PRPP is formed from ATP and D-ribose-5-phosphate (R5P) by the phosphoribosyl pyrophosphate synthetases (PRSs). The human PRS family, which has 3 isoforms (hPRS1, hPRS2 and hPRS3), belongs to the class I PRSs that requires divalent metal ions such as Mg2+ as the activator, inorganic phosphate ion for activity, and ATP or dATP as the diphosphoryl donor. Due to the important role of PRPP in the nucleotide metabolic process, the stability of PRPP content is essential for cell physiology and is predominantly controlled by hPRS1, the ubiquitously expressed human PRPP synthetase. Mutations in hPRS1 affect vital cell functions and are related to many diseases and disorders.

We determined the crystal structures of the E43T, D65N, A87T, M115T and Q133P mutations at a resolution of 3.0 Å, 2.14 Å, 3.3 Å, 2.11 Å and 2.74 Å, respectively, with 2 molecules in each asymmetric unit. Overall, the structures of all the five structures are highly similar to that of the wild type PRS1 with RMSD listed in S2 Table. In the A87T and M115T structures, the mutations of hydrophobic residues decrease the hydrophobic character of both Ala87 and Met115. In the PRS1 structure, Ala87 is located in the hydrophobic core of the N-terminal domain, whereas Met115 is located at the hydrophobic A-B dimer interface. Consequently, the M115T mutation might affect the A-B dimerization interface, whereas the A87T mutation might slightly affect the secondary structural elements of the N terminal domain. Nearly 13% of the mutations affect dimer interfaces directly, such as N114S and M115T. The N114S mutant decreases the hydrogen bond interaction whereas the M115T mutant reduces the residue’s hydrophobic interactions around the interface. These 2 mutations do not affect the protein structure, but may slightly decrease the protein’s aggregation states, thereby affects the protein’s regulation or catalytic efficiency.

>MPNIKIFSGSSHQDLSQKIADRLGLELGKVVTKKFSNQETCVEIGESVRGEDVYIVQSGCGEINDNLMELLIMINACKIASASRVTAVIPCFPYARQDKKDKSRAPISAKLVANTLSVAGADHIITMDLHASQIQGFFDIPVDNLYAEPAVLKWIRENISEWRNCTIVSPDAGGAKRVTSIADRLNVDFALIHKERKKANEVDRMVLVGDVKDRVAILVDDMADTCGTICHAADKLLSAGATRVYAILTHGIFSGPAISRINNACFEAVVVTNTIPQEDKMKHCSKIQVIDISMILAEAIRRTHNGESVSYLFSHVPLLEHHHHHH[2x]> AKDIEISASESKFILEALRQNYRLDGRSFDQFRDVEITFGKEFGDVSVKM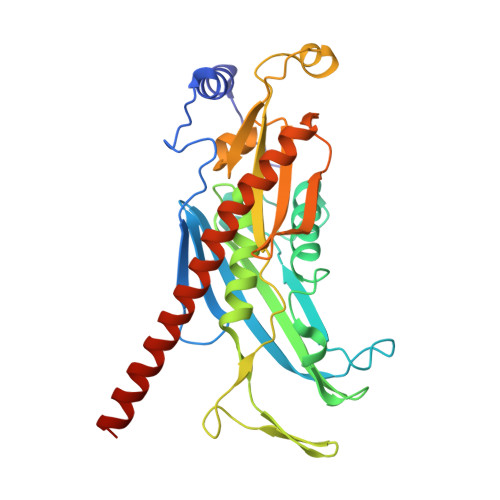GNTKVHCRISCQIAQPYEDRPFEGLFVISTEISPMAGSQFENGNITGEDEVLCSRIIEKSVRRSGALDVEGLCIVAGSKCWAVRADVHFLDCDGGFIDASCIAVMAGLMHFKKPDITVHGEQIIVHPVNEREPVPLGILHIPICVTFSFFNPQDTEENIKGETNSEISIIDATLKEELLRDGVLTVTLNKNREVVQVSKAGGLPMDALTLMKCCHEAYSIIEKITDQILQLLKEDSEKRNKYAAMLTSENAREI> ADELSTMSEPTITNHAQQQAQHLTNTELSSAESKSQDTSQITPKTNREKEQSQDLVSEPTTTELADTDAASMANTGPDATQKSASLPPVNTDIHDWVKTKGAWDKGYKGQGKVVAVIDTGIDPAHQSMRISDVSTAKVKSKEDMLARQKAAGINYGSWINDKVVFAHNYVENSDNIKENQKYESHGMHVTGIVAGNSKEAAATGERFLGIAPEAQVMFMRVFANDVMGSAESLFIKAIEDAVALGADVINLSLGTANGAQLSGSKPLMEAIEKAKKAGVSVVVAAGNERVYGSDHDDPLATNPDYGLVGSPSTGRTPTSVAAINSKWVIQRLMTVEELEKRADLNHGKAIYSESVDFKNIKDSLGYDKSHQFAYVKESTDAGYNAQDVKGKIALIERDPNKTYDEMIALAKKHGALGVLIFNNKPGQSNRSMRLTANGMGIPSAFISHEFGKAMSQLNGNGTGSLEFDSVVSKAPSQKGNEMNHFSNWGLTSDGYLKPDITAPGGDIYST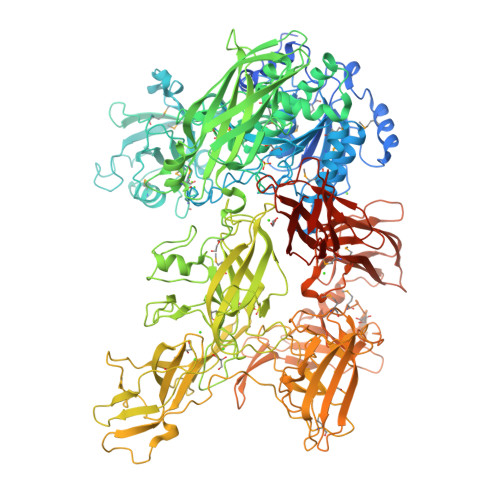YNDNHYGSQTGTSMASPQIAGASLLVKQYLEKTQPNLPKEKIADIVKNLLMSNAQIHVNPETKTTTSPRQQGAGLLNIDGAVTSGLYVTGKDNYGSISLGNITDTMTFDVTVHNLSNKDKTLRYDTELLTDHVDPQKGRFTLTSRSLKTYQGGEVTVPANGKVTVRVTMDVSQFTKELTKQMPNGYYLEGFVRFRDSQDDQLNRVNIPFVGFKGQFENLAVAEESIYRLKSQGKTGFYFDESGPKDDIYVGKHFTGLVTLGSETNVSTKTISDNGLHTLGTFKNADGKFILEKNAQGNPVLAISPNGDNNQDFAAFKGVFLRKYQGLKASVYHASDKEHKNPLWVSPESFKGDKNFNSDIRFAKSTTLLGTAFSGKSLTGAELPDGYYHYVVSYYPDVVGAKRQEMTFDMILDRQKPVLSQATFDPETNRFKPEPLKDRGLAGVRKDSVFYLERKDNKPYTVTINDSYKYVSVEDNKTFVERQADGSFILPLDKAKLGDFYYMVEDFAGNVAIAKLGDHLPQTLGKTPIKLKLTDGNYQTKETLKDNLEMTQSDTGLVTNQAQLAVVHRNQPQSQLTKMNQDFFISPNEDGNKDFVAFKGLENNVYNDLTVNVYAKDDHQKQTPIWSSQAGAGASAIESTAWYGITARGSKVMPGDYQYVVTYRDEHGKEHQKQYTISVNDKKPMITQGRFDTINGVDHFTPDKTKALGSSGIVREEVFYLAKKNGRKFDVTEGKDGITVSDNKVYIPKNPDGSYTISKRDGVTLSDYYYLVEDRAGNVSFATLRDLKAVGKDKAVVNFGLDLPVPEDKQIVNFTYLVRDADGKPIENLEYYNNSGNSLILPYGKYTVELLTYDTNAAKLESDKIVSFTLSADNNFQQVTFKMTMLATSQITAHFDHLLPEGSRVSLKTAQGQLIPLEQSLYVPKAYGKTVQEGTYEVVVSLPKGYRIEGNTKVNTLPNEVHELSLRLVKVGDASDSTGDHKVMSKNNSQALTASATPTKTTTPATAKA>[2x]GPLGSPNSQARPTVIRWSEGGKEVFISGSFNNWSTKIPLIKSHNDFVAILD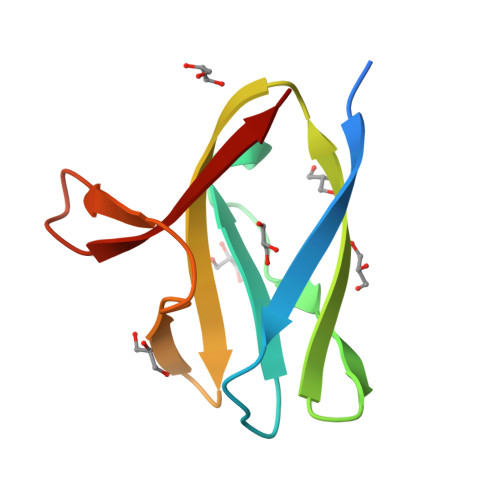LPEGEHQYKFFVDGQWVHDPSEPVVTSQLGTINNLIHVK>[2x]GPHMLKIADQSVDLNLKLMKWRILPDLNLDIIKNTKVLLLGAGTLGCYVSRALIAWGVRKITFVDNGTVSYSNPVRQALYNFEDCGKPKAELAAASLKRIFPLMDATGVKLSIPMIGHKLVNEEAQHKDFDRLRALIKEHDIIFLLVDSRESRWLPSLLSNIENKTVINAALGFDSYLVMRHGNRDEQSSKQLGCYFCHDVVAPTDSLTDRT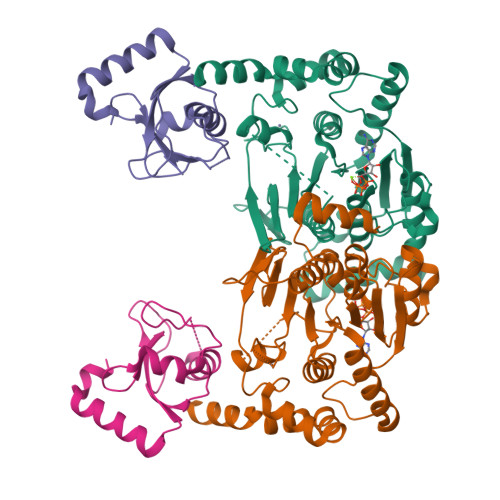LDQMCTVTRPGVAMMASSLAVELMTSLLQTKYSGSETTVLGDIPHQIRGFLHNFSILKLETPAYEHCPACSPKVIEAFTDLGWEFVKKALEHPLYLEEISGLSVIKQEVERLGNDVFEWEDDESDEIA;>GPHMKSTFKSEYPFEKRKAESERIADRFPNRIPVICEKAEKSDIPEIDKRKYLVPADLTVGQFVYVIRKRIMLPPEKAIFIFVNDTLPPTAALMSAIYQEHKDKDGFLYVTYSGENTFG[2x]>MSVGIVYGDQYRQLCCSSPKFGDRYALVMDLINAYKLIPELSRVPPLQWDSPSRMYEAVTAFHSTEYVDALKKLQMLHCEEKELTADDELLMDSFSLNYDCPGFPSVFDYSLAAVQGSLAAASALICRHCEVVINWGGGWHHAKRSEASGFCYLNDIVLAIHRLVSSTPPETSPNRQTRVLYVDLDLHHGDGVEEAFWYSPRVVTFSVHHASPGFFPGTGTWNMVDNDKLPIFLNGAGRGRFSAFNLPLEEGINDLDWSNAIGPILDSLNIVIQPSYVVVQCGADCLATDPHRIFRLTNFYPNLNLDSDCDSECSLSGYLYAIKKILSWKVPTLILGGGGYNFPDTARLWTRVTALTIEEVKGKKMTISPEIPEHSYFSRYGPDFELDIDYFPHESHNKTLDSIQKHHRRILEQLRNYADLNKLIYDYDQVYQLYNLTGMGSLVPR[4x]

Indeed, several studies have demonstrated the role of HDACs in the life cycle of Schistosoma; class I HDACs (smHDAC1, 3, and 8) were found to be expressed in all stages of Schistosoma lifecycle, with smHDAC8 showing the highest abundance. We showed that mice infected with schistosomula knocked down for smHDAC8 transcripts showed a decreased number of recovered adult worms and lower egg burden, suggesting that this enzyme is a valid therapeutic target. Therefore, small-molecule smHDAC8 inhibitors represented a promising approach for the treatment of schistosomiasis. SmHDACs, and in particular smHDAC8, warrant attention as they are validated targets and are of potentially high therapeutic value in the search of new small molecules for the treatment of schistosomiasis.

J1036, bearing an n-pentylhydroxamate group and an N-(4-chlorophenyl) substituent, showed the highest inhibitory potency against smHDAC8 among all tested compounds. To get molecular insight into the mode of action of the newly identified inhibitors bearing n-alkyl substituted hydroxamate moiety, the crystallographic structure of the complex between smHDAC8 and J1036 compound at 1.55 Å was determined and refined. The electron density for the inhibitor was not perfect but its binding at the catalytic zinc could be unambiguously assessed. We observed only part of the inhibitor structure in monomer B. Here, the hydroxamate is interacting with the zinc ion and the long alky chain is located in the foot pocket, indicating that the compound is partially hydrolyzed under the X-ray conditions. This is confirmed by the observed binding of the cleaved capping group of J1036 in a noncatalytic smHDAC8 pocket. Analysis of the crystal structure of the smHDAC8/J1036 complex in monomer A shows that the inhibitor binds in the smHDAC8 active-site pocket, where it forms specific interactions with the enzyme. The internal hydroxamate group is coordinating smHDAC8 catalytic zinc ion in a bidentate fashion. The n-pentyl-hydroxamate group additionally interacts via hydrogen bonding with three residues, namely His141, His142 and Tyr341. The J1036 n-pentyl moiety is deeply buried in the smHDAC8 foot-pocket, underneath the catalytic zinc ion, where it makes non-polar contacts with smHDAC8 residues Phe21, Trp140 and Cys152. Finally, the halogen-substituted phenyl capping group of J1036 forms parallel-displaced π–π stacking with Phe216.> PQFHLWKRPVVTAHIEGQPVEVLLDTGADDSIVTGIELGPHYTPKIVGGIGGFINTKEYKNVEIEVLGKRIKGTIMTGDTPINIFGRNLL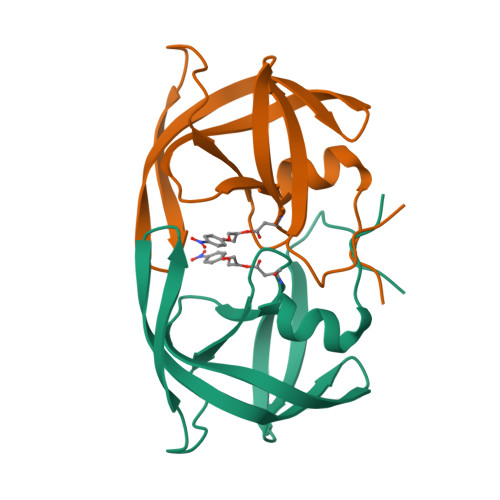TALGMSLNF> GAHMDCHLSDMLQQLHSVNASKPSERGLVRQEEAEDPACIPIFWVSKWVDYSDKYGLGYQLCDNSVGVLFNDSTRLILYNDGDSLQYIERDGTESYLTVSSHPNSLMKKITLLKYFRNYMSEHLLKAGANITPREGDELARLPYLRTWFRTRSAIIL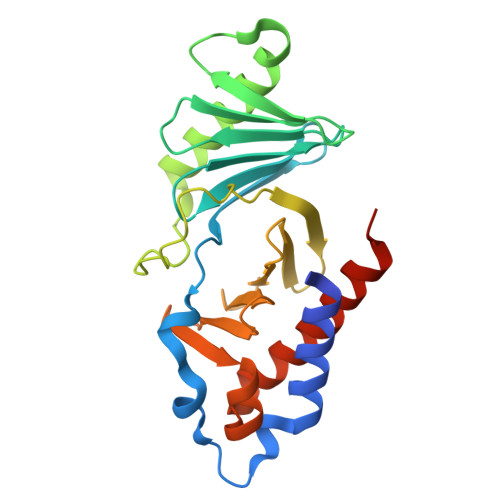HLSNGSVQINFFQDHTKLILCPLMAAVTYIDEKRDFRTYRLSLLEEYGCCKELASRLRYARTMVDKLLSSRSASNRLKA>[2x]HTSPLLAPVRQIHAFGDSYSDNGESQRLTREMLAKGIAGAQALPGEVYWQGRWSNGPTAVEVLARQLGAQLADHAVGGAKSGADNYYGWMSAYRHTGLAGQVDAYLATLDGKPVDGQALHFIFVSANDFFEHEDFAGEQPLEQLAGSSVANIRAAVQRLGEAGARRFLVVS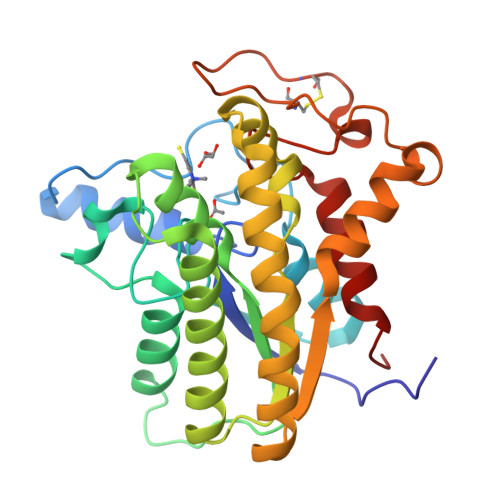STDLSVVPAVVAGNRVERAQRYLQAVNASLPIQLAALRKTRGLELSWFDHLTFSRHLRRNPARYGLVELDAPCQPTQPSVRPACANPDQYYFWDEWHPTRRVHQLAGEAMAARYAR> DDKRGRREIRVLHLLEQIRAYCETCWEWQEAHEPGMDQDKNPMPAPVEHQICPAVCVLMKLSFDEEHRHAMNELGGLQAIAELLQVDCEMYGLTNDHYSITLRRYAGMALTNLTFGDVANKATLCSMKGCMRALVAQLKSESEDLQQVIASVLRNLSWRADVNSKKTLREVGSVKALMECALEVKKESTLKSVLSALWNLSAHCTENKADICAVDGALAFLVGTLTYRSQTNTLAIIESGGGILRNVSSLIATNEDHRQ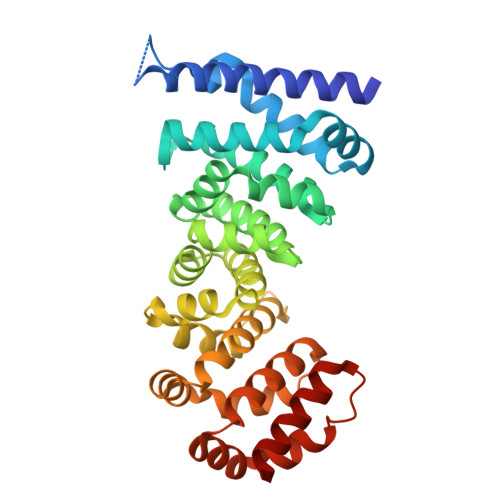ILRENNCLQTLLQHLKSHSLTIVSNACGTLWNLSARNPKDQEALWDMGAVSMLKNLIHSKHKMIAMGSAAALRNLMAN>[2x]AEQKTLHIYNWTDYIAPDTVANFEKETGIKVVYDVFDSNE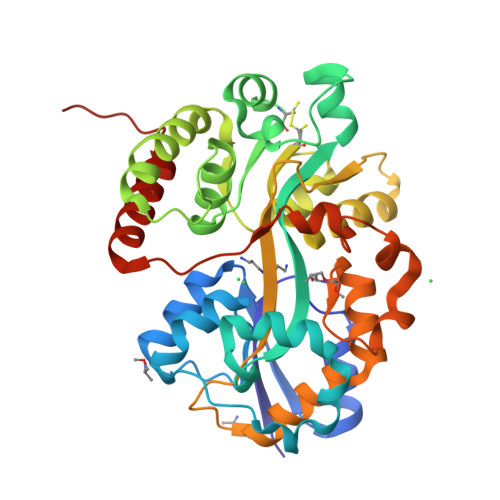VLEGKLMAGSTGFDLVVPSASYLERQLTAGVFQPLDKSKLPEWKNLDPELLKLVAKHDPDNKFAMPYMWATTGIGYNVDKVKAVLGENAPVDSWDLILKPENLEKLKSCGVSFLDDPEEVFATVLNYLGKDPNSTKADDYTGPATDLLLKLRPNIRYFHSSQYINDLANGDICVAIGWAGDVWQASNRAKEAKNGVNVSFSIPKEGAMAWFDVFAMPADAKNKDEAYQFLNYLLRPDVVAHISDHVFYANANKAATPLVSAEVRENPGIYPPADVRAKLFTQKVQDPKIDRVRTRAWTKVKSGKLEHHHHHH> SNAIQQSDGSMIIDGSANLRDLNKMFNWELDTEDARTFNGLILEHLEEIPDEG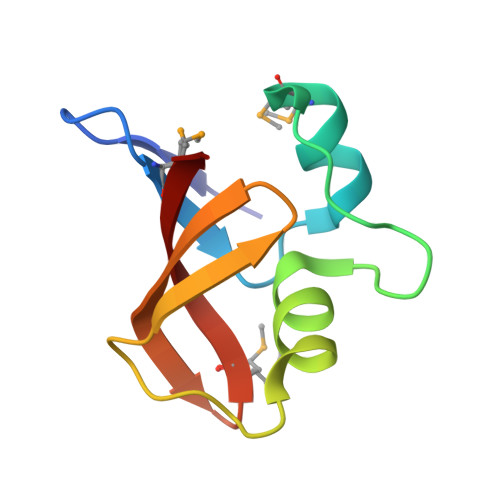TICEIDGLLITILEVGDNMIKQAKVVKL> MGLIQRRNFSTFASEPSVRFDFNYMKSVTPTTEEYYTYKSLFEVVPSTVPTLDESEPFKYAEIGHVSKNGEVFPVTLSFEDRDELNEDLFKKIEKGDIFLPERGNILISAIRPYLNKIVLIKEDDKTDIYFTKAFIQIKPLINSRILYYALRTIFSEKINAVSRQGKGYPTLKEDDLKTIQFSKKVIDNLLAKEEELISNIDALEKDIKELKSIQRSKKEIVDEVFSSHFNINMVELMALDSQRRVDVGLSSISSLNSTIRYSYRWNKMKLIQKYLYRDIDCIEPLGKYILSSNNGWSPESVVGGEGIPILGQEHLEFDGVLNVSPTKATTKTKNNMENFFIQEGDLFISRGNTVDLVGLACVVETEVTEDIIYPDLYIRLKIDEKVIHKKYLALLFNSFFGRLYFKYVSKGKNQTMVKISSNELLNYYLPIPPMEEQLEIVGK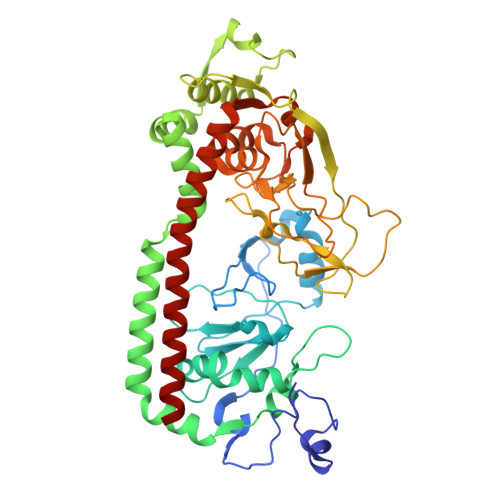IEEQIGAQNEIEKQIEEKRNQIRVIIEETARS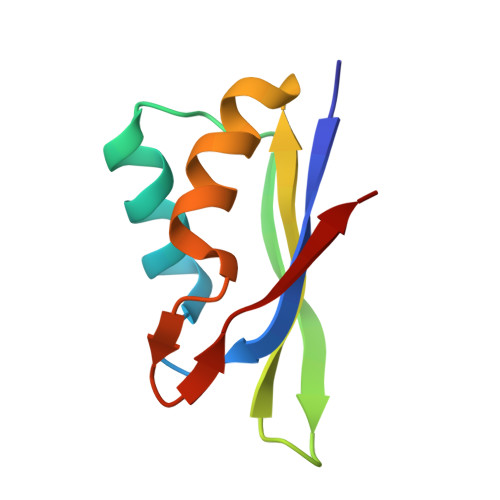> KISTLFLENLSAVCNKEFLKYLCHQENIRPFKIQIDGYDENSSTYSGFIKFRNFEDATRIFNFLNNRLVGGSIVTTSWE>MKHHHHHHSAGLEVLFQGPMEDGEVNDVVHPQVRAHINSLVSALGGISIDDDGGYKLGDDALEVLRDLKKWIRFYDEKTNRMDVARCLAEANIVSTDLLHILALWTPNENSNKYKARIALACFELMVPLTWPIEKDRETMTINHHRHIPVLQLAQLGYKRAIINYDAAPILSTAVRVALPAMAMPIGERTARDQGIIKLILYFLRNIAMITPPPGVKYEGDESQISRSALIDAFSYQDIFLTLLTIASNMGEDFRTEDVIVMEIIFHLVKRVDPKGQQLGSFVSDFLDSGFNPLFSHIRKSLEREAPHVLHYHQSQFFYLVAWFLEAERARRSSFNLIASVLTQE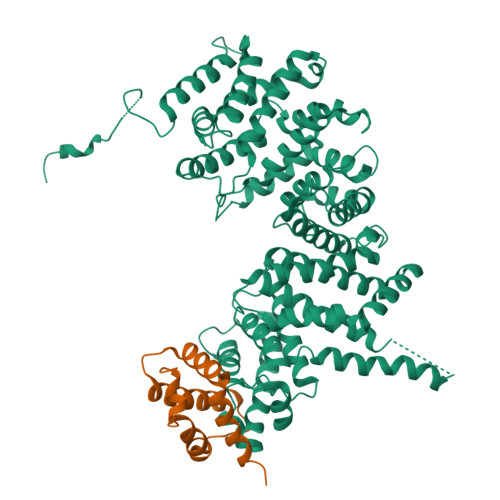MFIALNRALDRAYGDKDWRLLTSAMRCFTQILLTVQEMFDSGNDEDQEIADNILSRLFYEESTHDAVANIVRTYKDQGFEYLDACTELAHTFLRILEAYSKQNVDLQVRSGSADDEKMAEKTSQERKFDFKRFAARFTPQGVVDTFVTFTKYYRDLDDSQLKRAHRYFYRVAFKQEMSVMLFRLDIIHLFYNMIKGPEPLDKNSPMYKEWEELVRQILKRCIRKLEERPALFTEILFSKINSTAYYLEYGFEKQ[3x];>MTDALGIDKELNLKKKQRAPKVKLDDQRLLSEKGIPKLRKMAPRLKFKGKGHEFSDTARLLSFYQEWLDDLFPKATFLDALAMVEKAGHKTTVRNARLKWIDELRPKASFE[3x]(4aR,7aR)-6-(5-fluoropyrimidin-2-yl)-7a-(1,2-thiazol-5-yl)-4,4a,5,6,7,7a-hexahydropyrrolo[3,4-d][1,3]thiazin-2-amine 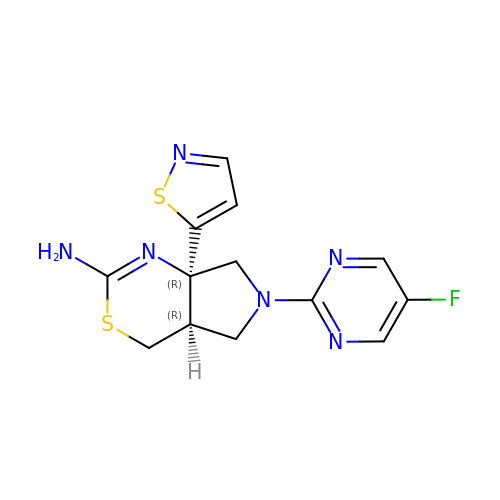| C13 H13 F N6 S2 | JTNSTOMSFFQQFP-SDBXPKJASA-N> ADQENSPLHTVGFDARFPQQNQTKHCWQSYVDYHKCVNMKGEDFAPCKVFWKTYNALCP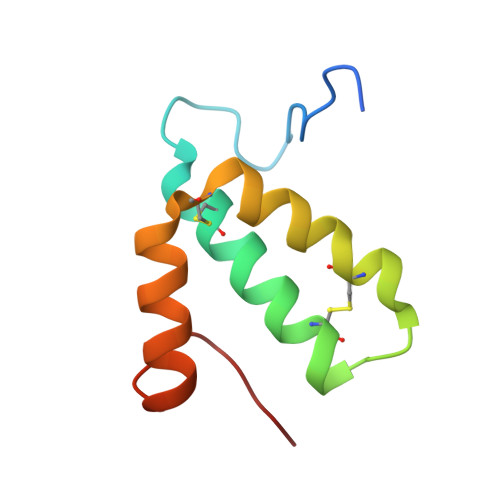LDWIEKWDDQREKGIFAGDINSD> D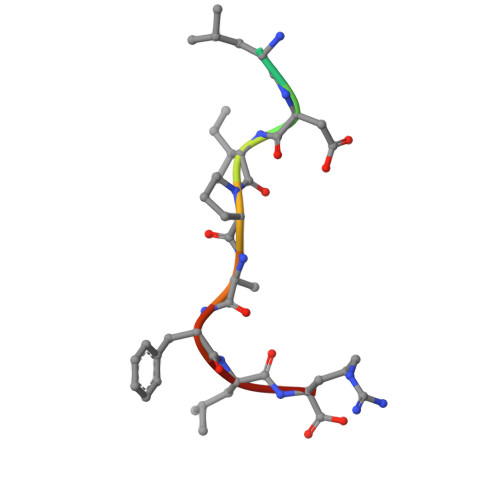YLDIPAFLR>GSMSSASTFGQNAWLVDEMFQQFQKDPKSVDKEWRELFEAQGGPNTTPATTEAQPSAPKESAKPAPKAAPAAKAAPRVETKPADKTAPKAKESSVPQQPKLPEPGQTPIRGIFKSIAKNMDISLEIPTATSVRDMPARLMFENRAMVNDQLKRTRGGKISFTHIIGYAMVKAVMAHPDMNNSYDVIDGKPTLIVPEHINLGLAIDLPQKDGSRALVVAAIKETEKMNFSEFLAAYEDIVARSRKGKLTMDDYQGVTVSLTNPGGIGTRHSVPRLTKGQGTIIGVGSMDYPAEFQGASEDRLAELGVGKLVTITSTYDHRVIQGAVSGEFLRTMSRLLTDDSFWDEIFDAMNVPYTPMRWAQDVPNTGVDKNTRVMQLIEAYRSRGHLIADTNPLSWVQPGMPVPDHRDLDIETHNLTIWDLDRTFNVGGFGGKETMTLREVLSRLRAAYTLKVGSEYTHILDRDERTWLQDRLEAGMPKPTQAEQKYILQKLNAAEAFENFLQTKYVGQKRFSLEGAEALIPLMDSAIDTAAGQGLDEVVIGMPHRGRLNVLFNIVGKPLASIFNEFEGQMEQGQIGGSGDVKYHLGSEGQHLQMFGDGEIKVSLTANPSHLEAVNPVMEGIVRAKQDYLDKGVDGKTVVPLLLHGDAAFAGLGIVPETINLAKLRGYDVGGTIHIVVNNQIGFTTTPDSSRSMHYATDYAKAFGCPVFHVNGDDPEAVVWVGQLATEYRRRFGKDVFIDLVCYRLRGHNEADDPSMTQPKMYELITGRETVRAQYTEDLLGRGDLSNEDAEAVVRDFHDQMESVFNEVKEGGKKQAEAQTGITGSQKLPHGLETNISREELLELGQAFANTPEGFNYHPRVAPVAKKRVSSVTEGGIDWAWGELLAFGSLANSGRLVRLAGEDSRRGTFTQRHAVAIDPATAEEFNPLHELAQSKGNNGKFLVYNSALTEYAGMGFEYGYSVGNEDSIVAWEAQFGDFANGAQTIIDEYVSSGEAKWGQTSKLILLLPHGYEGQGPDHSSARIERFLQLCAEGSMTVAQPSTPANHFHLLRRHALSDLKRPLVIFTPKSMLRNKAAASAPEDFTEVTKFQSVINDPNVADAAKVKKVMLVSGKLYYELAKRKEKDGRDDIAIVRIEMLHPIPFNRISEALAGYPNAEEVLFVQDEPANQGPWPFYQEHLPELIPNMPKMRRVSRRAQSSTATGVAKVHQLEEKQLIDEAFEA[6x];>[6x]GMSDNNGTPEPQVETTSVFRADLLKEMESSTGTAPASTGAENLPAGSALLVVKRGPNAGARFLLDQPTTTAGRHPESDIFLDDVTVSRRHAEFRINEGEFEVVDVGSLNGTYVNREPRNAQVMQTGDEIQIGKFRLVFLAGPAE

Contrary to most organisms in which three enzymes compose the 2-oxoglutarate dehydrogenase complex (ODH), actinobacteria rely on a two-in-one protein (OdhA) in which both the oxidative decarboxylation and succinyl transferase steps are carried out by the same polypeptide. Here we describe high-resolution cryo-EM and crystallographic snapshots of representative enzymes from Mycobacterium smegmatis and Corynebacterium glutamicum, showing that OdhA is an 800-kDa homohexamer that assembles into a three-blade propeller shape. The obligate trimeric and dimeric states of the acyltransferase and dehydrogenase domains, respectively, are critical for maintaining the overall assembly, where both domains interact via subtle readjustments of their interfaces. Schematic illustration of the reaction steps involved in the oxidative decarboxylation of 2-oxoglutarate with generation of succinyl-CoA and NADH/H+ (ODH reaction), with emphasis on the catalytic steps catalyzed by OdhA. These include the ThDP-dependent decarboxylation of the 2-oxoglutarate substrate followed the reductive acylation of the lipoyl group provided by E2p (both catalyzed by the OdhA E1o domain), and the transfer of the succinyl moiety to the CoASH acceptor (catalyzed by the OdhA E2o domain).

By preincubating purified OdhA with an excess OdhI and passing the sample through size exclusion chromatography prior to grid preparation, we were also able to obtain a single particle reconstruction of a full OdhA-OdhI complex at 2.3 Å resolution. The overall structure is very similar to that of the homologous MsKGD-GarA complex, with OdhI molecules binding, through their FHA domains (traceable for residues Glu40-Ala142), to the OdhA E1o domain with a 1:1 stoichiometry. In contrast to the other single particle EM structures, OdhA adopts here the resting conformation, equivalent to the one observed in the crystal structure of OdhAΔ97 and consistently with structural and kinetic observations on mycobacterial KGD, both indicating that GarA binding stabilized this enzyme conformation. Moreover, no ligand bound to the OdhA acetyl-CoA allosteric site could be detected in this complex, suggesting that bound acetyl-CoA may have been lost because of OdhI binding, further confirming the link between the presence of the activator and the conformational state of the enzyme. Interactions with OdhA involve the tips of both OdhI FHA antiparallel β-sheets: one anchors firmly to the OdhA loop Leu591-Glu598, which connects two antiparallel β-strands, while the tip of the other OdhI β-sheet binds the OdhA α-helices Gln480-Lys503 and Asn786-Asn805 (αE). Most notably, no hydrogen bond was observed between the phosphomimetic residue Asp795 in OdhA and OdhI Ser86, in contrast to structural observations on the GarA-MsKGD complex but consistently with site-directed mutagenesis on OdhI, which pointed to Ser86 as dispensable for binding.In this context, we recently reported the characterization of a novel xyloglucan utilization locus (XyGUL) that confers Bacteroides ovatus, and species harbouring syntenic XyGULs, with the ability to utilize this abundant vegetable polysaccharide across sampled human populations. Here, we present the three-dimensional structures of BoGH31, BoGH43A, BoGH43B and BoGH3B, expanding our knowledge of the structural determinants required for xyloglucan degradation. Our analyses highlight key adaptations in these enzymes that confer their specificity for xyloglucan oligosaccharides, while also providing a rationale for the maintenance of two divergent genes coding for GH3 enzymes, and similarly two divergent genes for GH43 family members, within the same PUL. While we were unable to determine a structure for BoGH3A, our structural and sequence analysis of BoGH3B has also allowed us to highlight further potential differences between these two enzymes encoded by the operon. Together with existing biochemical data, our analyses of the three-dimensional structures, and various enzyme-inhibitor complexes, of BoGH31, BoGH43A, BoGH43B and BoGH3B provide molecular-level insight into the stepwise breakdown of xyloglucan by the BoXyGUL.

There are two GH43 family members represented in the B. ovatus xyloglucan PUL: BoGH43A and BoGH43B. Both enzymes have demonstrable activity on l-Araf-α-PNP, though BoGH43A was considerably more active, and both are thought to be responsible for the removal of pendant arabinofuranoside side chains from solanaceous xyloglucan substrates, thereby converting S to X for further processing by the α-xylosidase and other members of the PUL. Crystals of BoGH43A in complex with AraDNJ and AraLOG were obtained by soaking native crystals in 10 mM (final) solutions of respective compounds supplemented with mother liquor for 60 min, prior to cryocooling. Soaking of native BoGH43A with two putative inhibitors, AraDNJ and AraLOG, yielded respective enzyme–ligand complexes, confirming this as the active site. AraDNJ was able to displace TRIS from the −1 sub-site and appeared bound in a low-energy 3E conformation typical of iminosugar ‘furanose’ inhibitors. The side-chain carboxylate of Asp140 (O3 and O4 positions), the backbone amino group of Ala94 (O4) and the OD2 atom of Asp34 all directly coordinated the inhibitor. GH43 members typically contain three highly conserved acidic residues in their active sites to impart activity. Together with Asp34 as the general base, which activates water to attack the anomeric carbon, Glu189 is ideally poised as the general acid, while Asp140 completes the triplet of residues and is important for modulating the pKa and orienting the general acid for catalysis. AraDNJ binds to BoGH43A with Kd = 35 ± 4 µM, while AraLOG binding was too weak to be measured using this technique, consistent with its inability to displace TRIS during crystal soaking.

>[2x]MGSSHHHHHHQGYSNPVIPGFHPDPSVCKAGDDYYLVNSSFQYFPGVPLFHSKDLVHWEQIGNCLTRPSQLDLTNANSGSGIFAPTIRYNDGVFYMITTNVSGKGNFLVHTTDPRSEWSEPVWLEQGGIDPSLYFEDGKCFMVSNPDGYINLCEIDPMTGKQLSSSKRIWNGTGGRYAEGPHIYKKDGWYYLLISEGGTELGHKVTIARSRYIDGPYQGNPANPILTHANESGQSSPIQGTGHADLVEGTDGSWWMVCLAYRIMPGTHHTLGRETYLAPVRWDKDAWPVVNSNGTISLKMDVPTLPQQEMKGRPERIDFKEGKLSPEWIHLQNPEAKNYIFTKDGKLRLIATPVTLSDWKSPTFVALRQEHFDMEASAPVVLQKAGVNDEAGISVFMEFHSHYDLFVRQDKDRKRSVGLRYKLGEITHYAKEVSLPTDGEVELVVKSDINYYYFGYKVNGIYHDLGKMNTRYLSTETAGGFTGVVLGLYITSASKDSKAYADFEYFKYKGKPGENK> GLPTKPGPGSYQFMTTDED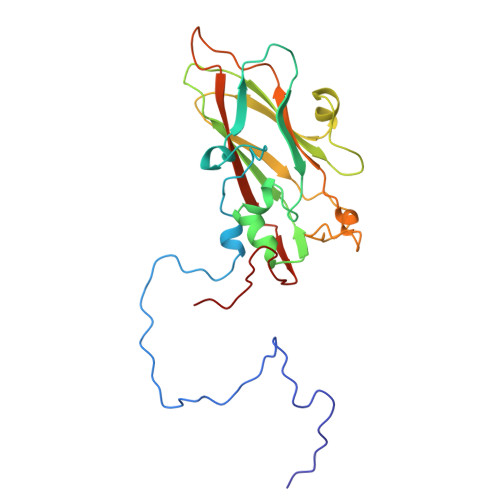CSPCILPDFQPTPEIFIPGKVNNLLEIAQVESILEANNREGVEGVERYVIPVSVQDALDAQIYALRLELGGSGPLSSSLLGTLAKHYTQWSGSVEITCMFTGTFMTTGKVLLAYTPPGGDMPRNREEAMLGTHVIWDFGLQSSITLVIPWISASHFRGVSNDDVLNYQYYAAGHVTIWYQTNMVIPPGFPNTAGIIMMIAAQPNFSFRIQKDREDMTQTAILQ>MKHSLPDLPYDYGALEPHINAQIMQLHHSKVHAAYVNNLNVTEEKYQEALAKGDVTAQIALQPALKFNGGGHINHSIFWTNLSPNGGGEPKGELLEAIKRDFGSFDKFKEKLTAASVGVQGSGWGWLGFNKERGHLQIAACPNQDPLQGTTGLIP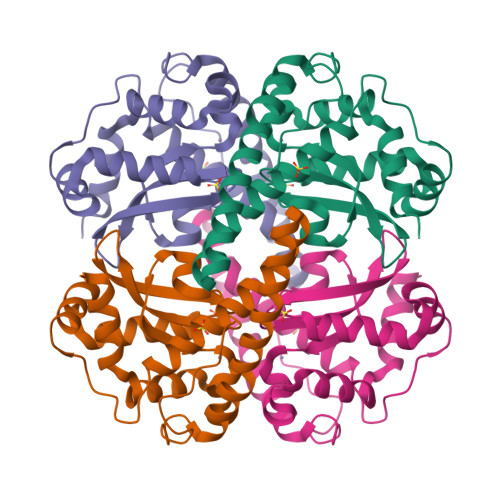LLGIDVWEHAYYLQYKNVRPDYLKAIWNVINWENVTERYMACKK[2x]> ERYENLFAQLNDRREGAFVPFVTLGDPGIEQSLKIIDTLIDAGADALELGVPFSDPLADGPTIQNANLRAFAAGVTPAQCFEMLALIREKHPTIPIGLLMYANLVFNNGIDAFYARCEQVGVDSVLVADVPVEESAPFRQAALRHNIAPIFICPPNADDDLLRQVASYGRGYTYLLSRSGVTGAENRGALPLHHLIEKLKEYHAAPALQGFGISSPEQVSAAVRAGAAGAISGSAIVKIIEKNLASPKQMLAELRSFVSAMKAASR;> TLLNPYFGEFGGMYVPQILMPALNQLEEAFVSAQKDPEFQAQFADLLKNYAGRPTALTKCQNITAGTRTTLYLKREDLLHGGAHKTNQVLGQALLAKRMGKSEIIAETGAGQHGVASALASALLGLKCRIYMGAKDVERQSPNVFRMRLMGAEVIPVHSGSATLKDACNEALRDWSGSYET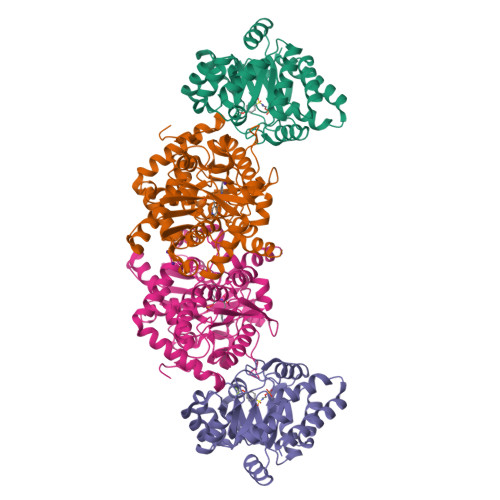AHYMLGTAAGPHPYPTIVREFQRMIGEETKAQILDKEGRLPDAVIACVGGGSNAIGMFADFINDTSVGLIGVEPGGHGIETGEHGAPLKHGRVGIYFGMKAPMMQTADGQIEESYSISAGLDFPSVGPQHAYLNSIGRADYVSITDDEALEAFKTLCRHEGIIPALESSHALAHALKMMREQPEKEQLLVVNLSGRGDKDIFTVHDILKA>M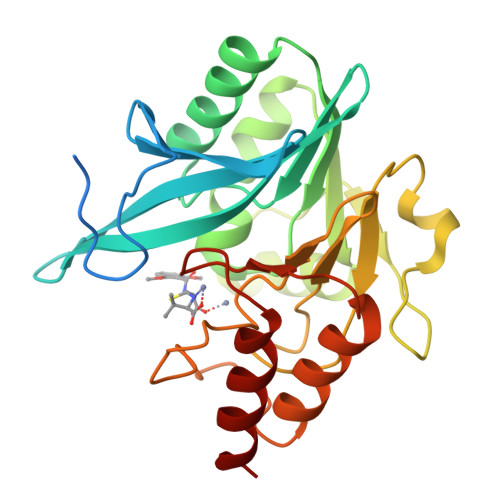ELPNIMHPVAKLSTALAAALMLSGCMPGEIRPTIGQQMETGDQRFGDLVFRQLAPNVWQHTSYLDMPGFGAVASNGLIVRDGGRVLVVDTAWTDDQTAQILNWIKQEINLPVALAVVTHAHQDKMGGMDALHAAGIATYANALSNQLAPQEGMVAAQHSLTFAANGWVEPATAPNFGPLKVFYPGPGHTSDNITVGIDGTDIAFGGCLIKDSKAKSLGNLGDADTEHYAASARAFGAAFPKASMIVMSHSAPDSRAAITHTARMADKLR[2x]>[2x]MSASDALNSCPHVALLLSSGMGHLTPCLRFAATLVQHHCRVTIITNYPTVSVAESRAISLLLSDFPQITEKQFHLLPFDPSTANTTDPFFLRVEAIRRSAHLLNPLLSSISPPLSALVIDSSLFSSFVPVAANLDLPSYVLFTSSTRMCSLEETFPAFVASKTNFDSIQLDDVIEIPGFSPVPVSSVPPVALNLNHLFTTMLIQNGQSFRKA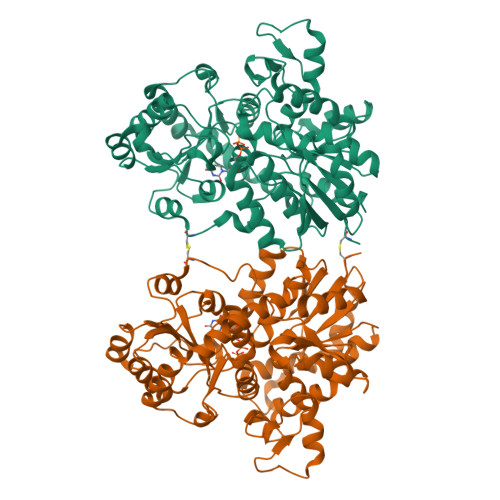NGILINTFEALEGGILPGINDKRAADGLPPYCSVGPLLPCKFEKTECSAPVKWLDDQPEGSVVYVSFGSHFALSSEQIKELGDGLIRSGCRFLWVVKCKKVDQEDEESLDELLGRDVLEKIKKYGFVIKNWVNQQEILDHRAVGGFVTHGGWNSSMEAVWHGVPMLVWPQFGDQKINAEVIERSGLGMWVKRWGWGTQQLVKGEEIGERIKDLMGNNPLRVRAKTLREEARKAIEVGGSSEKTLKELIENWKKTSRKT>[4x]MSDSHHKPVWDRTHHAKMATGIGDPQCFKGMAGKSKFNVGDRVRIKDLPDLFYTRTMTYTRGATGTIVRLVYESPAAEDEAFGNEENVEWFYSIVFAQKDLWPEYSDTFANDTLETEIPERYLEKA;>MSSSIREEVHRHLGTVALMQPALHQQTHAPAPTEITHTLFRAYTRVPHDVGGEADVPIEYHEKEEEIWELNTFATCECLAWRGVWTAEERRRKQNCDVGQTVYLGMPYYGRWLLTAARILVDKQFVTLTELHNKIVEMRERVASGQGLGEYLPPKAK[4x];>[4x]MSADH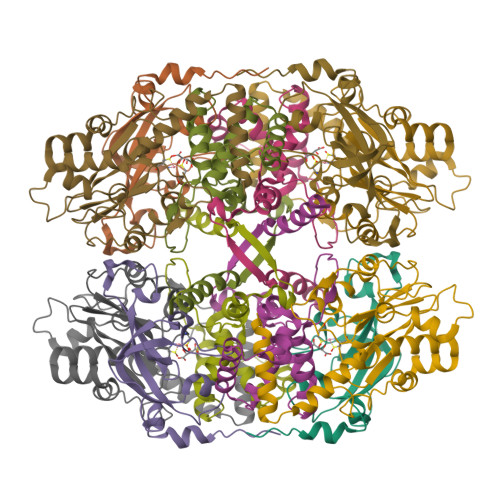DHDHDHDHDHKPAPMVEEVSDFEILEMAVRELAIEKGLFSAEDHRVWKDYVHTLGPLPAARLVAKAWLDPEYKKLCIEDGVEASKAVGVNWVTSPPTQFGTPSDYCNLRVLADSPTLKHVVVCTLCSCYPRPILGQSPEWYRSPNYRRRLVRWPRQVLAEFGLQLPSEVQIRVADSNQKTRYIVMPVRPEGTDGWTEDQLAEIVTRDCLIGVAVPKPGITVNAKRPVLKANRPVHHDH>GELVRTDSPNFLCSVLPTHWRCNKTLPIAFKVVAKGDVPDGTLVTVMAGNDENYSAELRNATAAMKNQVARFNDLRFVGRSGRGKSFTLTITVFTNPPQVATYHRAIKITGDGPREPRRHRQKLDDQTKPGSLSFSERLSELEQLRRTAMRVSPHHPAPTPNPRASLNHSTAFNPQPQSQMQDARQIQPSPPWSYDQSYQYLGS[2x];>[2x]MPRVVPDQRSKFENEEFFRKLSRECEIKYTGFRDRPHEERQTRFQNACRDGRSEIAFVATGTNLSLQFFPASWQGEQRQTPSREYVDLEREAGKVYLKAPMILNGVCVIWKGWIDLHRLDGMGCLEFDEERAQQEDALAQQA;>SLQRVPSYDSFDSEDYPAALPNHKPKGTFKDYVRDRADLNKDKPVIPAAALAGYTGSGPIQLWQFLLELLTDKSCQSFISWTGDGWEFKLSDPDEVARRWGKRKNKPKMN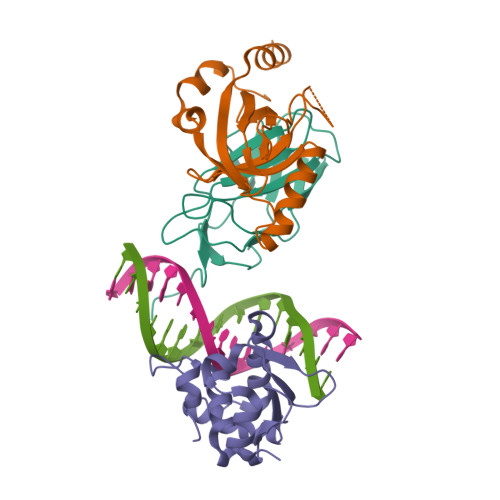YEKLSRGLRYYYDKNIIHKTAGKRYVYRFVCDLQSLLGYTPEELHAMLDVKPDADE[2x]>[4x]MGGHHHHHHGENLYFQGISSETGEMGILWEFDPIINKWIRLSMKLKVERKPFAEGALREA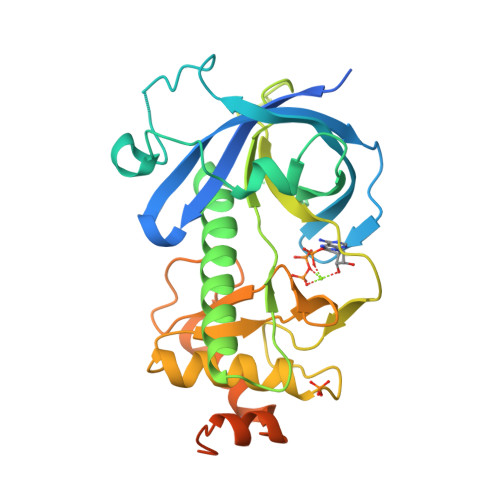YHTVSLGVGTDENYPLGTTTKLFPPIEMISPISKNNEAMTQLKNGTKFVLKLYKKEAEQQASRELYFEDVKMQMVCRDWGNKFNQKKPPKKIEFLMSWVVELIDRSPSSNGQPILCSIEPLLVGEFKKNNSNYGAVLTNRSTPQAFSHFTYELSNKQMIVVDIQGVDDLYTAPQIHTPDGKGFGLGNLGKAGINKFITTHKCNAVCALLDLDVKLGGVLSGNNKKQLQQGTMVMPDILPELMPSDNT>[10x]MQTTVTTMLLASVALAACAGGGSTPLPLPQQQPPQQEPPPPPVPLASRAACEALKDGNGDMVWPNAATVVEVAAWRDAAPATASAAALPEHCEVSGAIAKRTGIDGYPYEIKFRLRMPAEWNGRFFMEGGSGTNGSLSAATGSIGGGQIASALSRNFATIATDGGHDNAVNDNPDALGTVAFGLDPQARLDMGYNSYDQVTQAGKAAVARFYGRAADKSYFIGCSEGGREGMMLSQRFPSHYDGIVAGAPGYQLPKAGISGAWTTQSLAPAAVGLDAQGVPLINKSFSDADLHLLSQAILGTCDALDGLADGIVDNYRACQAAFDPATAANPANGQALQCVGAKTADCLSPVQVTAIKRAMAGPVNSAGTPLYNRWAWDAGMSGLSGTTYNQGWRSWWLGSFNSSANNAQRVSGFSARSWLVDFATPPEPMPMTQVAARMMKFDFDIDPLKIWATSGQFTQSSMDWHGATSTDLAAFRDRGGKMILYHGMSDAAFSALDTADYYERLGAAMPGAAGFARLFLVPGMNHCSGGPGTDRFDMLTPLVAWVERGEAPDQISAWSGTPGYFGVAARTRPLCPYPQIARYKGSGDINTEANFACAAPPLEHHHHHH

PETase cleaves BHET to MHET and EG, and the soluble MHET product is further hydrolyzed by MHETase to produce TPA and EG. Overall, the structure of MHETase is most similar to that of FAEs. The structural conservation between the hydrolase domains of MHETase and PETase is striking, and despite the large insertion of ∼240 residues representing the lid domain, residues Ser225, Asp492, and His528 effectively reconstitute the catalytic triad.

A similar Ca2+ binding site was characterized for Aspergillus oryzae FaeB (AoFaeB), wherein it was hypothesized to have a role in stabilizing the lid domain. To examine the effect of calcium binding, a fifth scenario absent of either MHET or Ca2+ was modeled in triplicate 150-ns simulations (the prior four scenarios each include bound Ca2+). These trajectories show evidence for lid stabilization upon Ca2+ binding mainly in the immediate vicinity of the calcium binding site. In fact, the terminal residues of the lid domain converge to within hydrogen-bonding distance of each other (Tyr252-Ala469, 2.9 Å), creating a compact linkage to the hydrolase domain. The lid domain of MHETase is exceptionally large, as average lid domains in α/β-hydrolases tend to be ∼100 residues, and is more typical of a lid from tannase family members (vide infra). One of the MHETase disulfides is located at the active site, connecting cysteines (Cys224 and Cys529) adjacent to the catalytic residues (Ser225 and His528, respectively), which is conserved in tannase family members.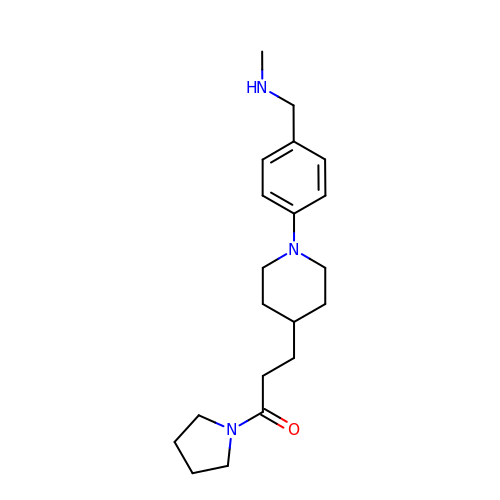3-[1-[4-(methylaminomethyl)phenyl]piperidin-4-yl]-1-pyrrolidin-1-yl-propan-1-one | C20 H31 N3 O | VOLHWJLFFDGPRY-UHFFFAOYSA-N> MALLAEHLLRPLPADKQIETGPFLEAVSHLPPFFDCLGSPVFTPIKADISGNITKIKAVYDTNPTKFRTLQNILEVEKEMYGAEWPKVGATLALMWLKRGLRFIQVFLQSICDGERDENHPNLIRVNATKAYEMALKKY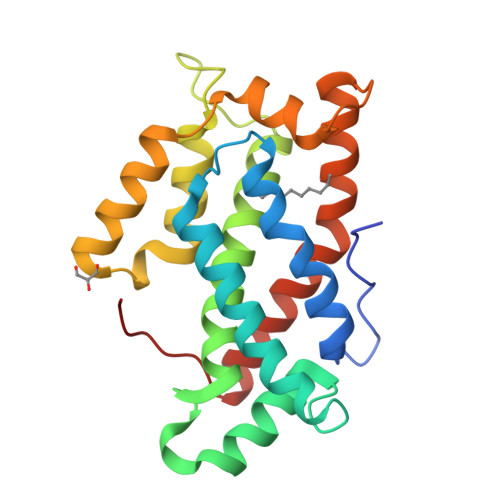HGWIVQKIFQAALYAAPYKSDFLKALSKGQNVTEEECLEKVRLFLVNYTATIDVIYEMYTRMNAELNYKV5-cyclohexyl-1,3-dihydroindol-2-one | 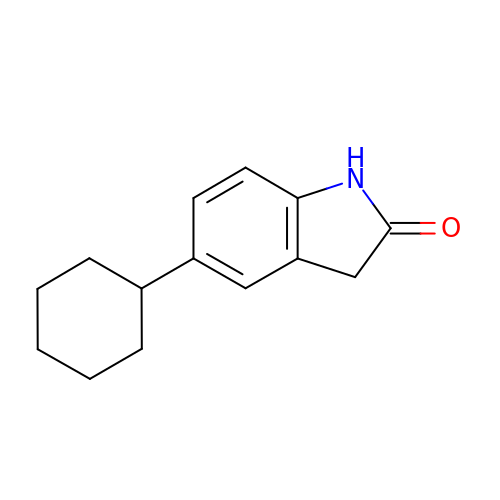C14 H17 N O | GAMOWVPYWCFRMK-UHFFFAOYSA-N>PNYKLTYFNMRGRAEIIRYIFAYLDIQYEDHRIEQADWPEIKSTLPFGKIPILEVDGLTLHQSLAIARYLTKNTDLAGNTEMEQCHVDAIVDTLDDFMSCFPWAEKKQDVKEQMFNELLTYNAPHLMQDLDTYLGGREWLIGM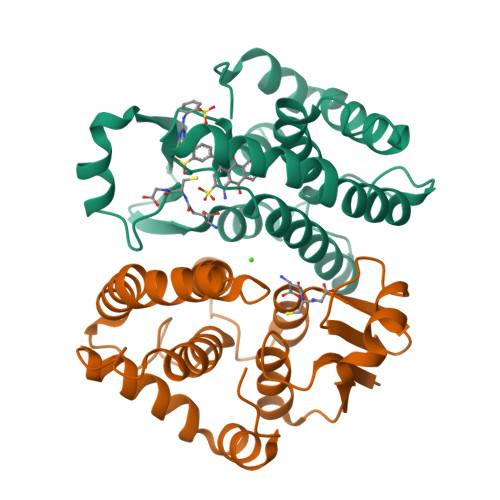SVTWADFYWEICSTTLLVFKPDLLDNHPRLVTLRKKVQAIPAVANWIKRRPQTKL[4x]>[4x]SMKQQKNSKGSSDFCVKNIKQAEFGRREIEIAEQEMPAL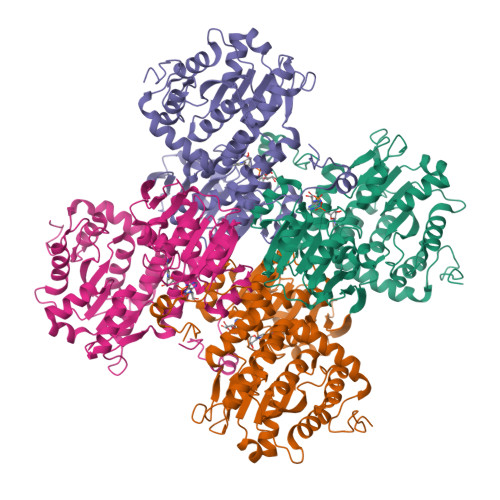MALRKRAQGEKPLAGAKIVGCTHITAQTAVLMETLGALGAQCRWAACNIYSTLNEVAAALAESGFPVFAWKGESEDDFWWCIDRCVNVEGWQPNMILDDGGDLTHWIYKKYPNMFKKIKGIVEESVTGVHRLYQLSKAGKLCVPAMNVNDSVTKQKFDNLYCCRESILDGLKRTTDMMFGGKQVVVCGYGEVGKGCCAALKAMGSIVYVTEIDPICALQACMDGFRLVKLNEVIRQVDIVITCTGNKNVVTREHLDRMKNSCIVCNMGHSNTEIDVASLRTPELTWERVRSQVDHVIWPDGKRIVLLAEGRLLNLSCSTVPTFVLSITATTQALALIELYNAPEGRYKQDVYLLPKKMDEYVASLHLPTFDAHLTELTDEQAKYLGLNKNGPFKPN>[5x]MNRRVLVTGATGLLG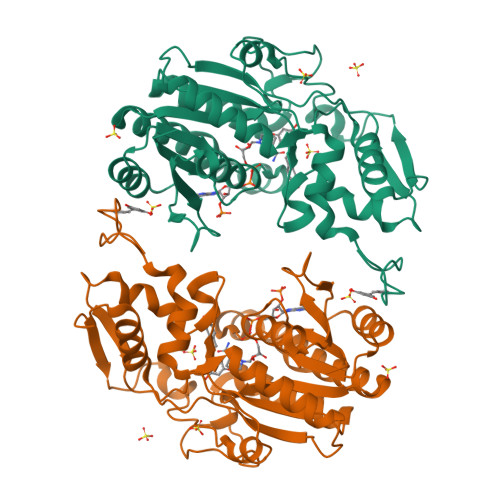RAVHKEFQQNNWHAVGCGFRRARPKFEQVNLLDSNAVHHIIHDFQPHVIVHCAAERRPDVVENQPDAASQLNVDASGNLAKEAAAVGAFLIYISSDYVFDGTNPPYREEDIPAPLNLYGKTKLDGEKAVLENNLGAAVLRIPILYGEVEKLEESAVTVMFDKVQFSNKSANMDHWQQRFPTHVKDVATVCRQLAEKRMLDPSIKGTFHWSGNEQMTKYEMACAIADAFNLPSSHLRPITDSPVLGAQRPRNAQLDCSKLETLGIGQRTPFRIGIKESLWPFLIDKRWRQTVFHAENLYFQ> AYEDSET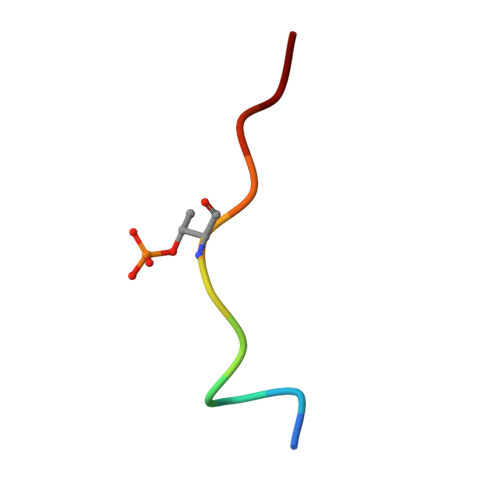QPFD>SNAMKIGIVGAMAQEVEILKNLMTERTETRVASAVIFEGKINGKDIALLQSGIGKVAAAIGTTALLQLAKPDCVINTGSAGGVAKGLKVGDIVISDETRYHDADVTAFGYEKGQLPANPAAFLSDKKLADLAQEMAEKQG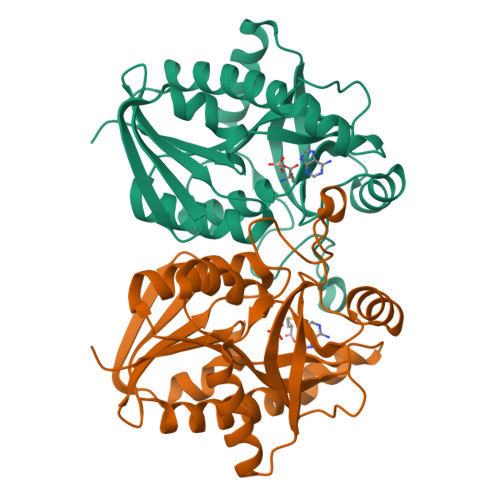QSVKRGLICSGDSFINSEDKIAQIQADFPNVMGVEMEATAIAQVCYAFNVPFVVVRAISDGGDGKASISFEEFLPLAAKQSSALVLEMIDRLSS[6x]> IVEKSKICSSRYEPTVRIGGRDGMCVDVYDNGYHNGNRIIMWKCKDRLEENQLWTLKSDKTIRSNGKCLTTYGYAPGSYVMIYDCTSAVAEATYWEIWDNGTIINPKSALVLSAESSSMGGTLTVQTNEYLMRQGWRTGNNTSPFVTSISGYSDLCMQAQGSNVWMADCDSNKKEQQWALYTDGSIRSVQNTNNCLTSKDHKQGSTILLMGCSNGWASQRWVFKNDGSIYSLYDDMVMDVKGSDPSLKQ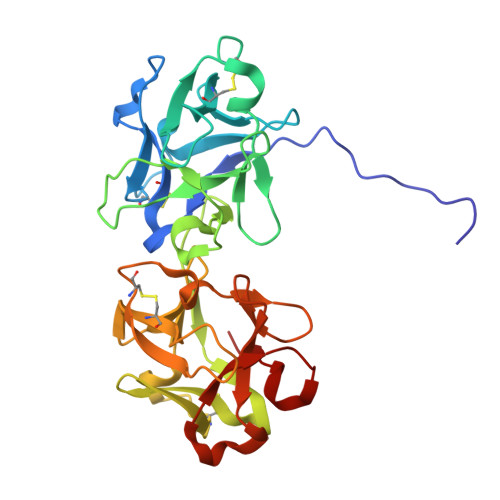IILWPYTGKPNQIWLTLF Tick-borne encephalitis virus (TBEV) is a member of the Flavivirus genus, and belongs in the family Flaviviridae. The TBEV virion consists of three structural proteins, the envelope (E), membrane (M), and capsid (C) proteins, and a positive-sense single-stranded RNA genome. The NC is covered by the viral envelope that consists of host-derived lipids into which 180 copies of both M and E are embedded. The fundamental building block of the virion is a heterotetramer made up of two M–E dimers.

Here, we present the structure of a low-passage, European TBEV subtype (Kuutsalo-14) solved with cryo-EM and single-particle reconstruction to a resolution of 3.3 Å. The merged K3 datasets gave a final reconstruction with a resolution of 3.3 Å. The asymmetric unit contains three E–M heterodimers. Superimposition of the three E–M heterodimers within the asymmetric unit, based on the E protein ectodomains, indicated conformational differences between the M proteins located on the two-fold (chain D), three-fold (chain E), and five-fold (chain F) symmetry axes. The major conformational differences between the three M proteins arise due to the different locations of Asp23 and Ser24 that diverge by up to 2.8 Å at the Cα. Chains D and F twist towards each other and interact at the heterotetramer interfaces within the raft. One π-stacking interaction between Trp37 on each M protein, and two salt bridges between Lys40 and Glu33 stabilise the M protein interface. For each E–M dimer within the asymmetric unit, the reconstruction contained two densities not accounted for by the protein model. As phosphatidylcholine (PC) is the most common lipid species found in flavivirus virions, we built PC headgroups and the first four carbon atoms of each fatty acid tail. We built two N-acetylglucosamines (GlcNac) with core fucosylation (Fuc) at the first GlcNac into the density, which is consistent with the TBEV glycome and with previous flavivirus structures.

>SRCTHLENRDFVTGTQGTTRVTLVLELGGCVTITAEGKPSMDVWLDAIYQENPAKTREYCLHAKLSDTKVAARCPTMGPATLAEEHQGGTVCKRDQSDRGWGNHCGLFGKGSIVACVKAACEAKKKATGHVYDANKIVYTVKVEPHTGDYVAANETHSGRKTASFTVSSEKTILTMGEYGDVSLLCRVASGVDLAQTVILELDKTVEHLPTAWQVHRDWFNDLALPWKHEGAQNWNNAERLVEFGAPHAVKMDVYNLGDQTGVLLKALAGVPVAHIEGTKYHLKSGHVTCEVGLEKLKMKGLTYTMCDKTKFTWKRAPTDSGHDTVVMEVTFSGTKPCRIPVRAVAHGSPDVNVAMLITPNPTIENNGGGFIEMQLPPGDNIIYVGELSHQWFQKGSSIGRVFQKTKKGIERLTVIGEHAWDFGSAGGFLSSIGKAVHTVLGGAFNSIFGGVGFLPKLLLGVALAWLGLNMRNPTMSMSFLLAGGLVLAMTLGVGA[3x];>[3x]SVLIPSHAQGELTGRGHKWLEGDSLRTHLTRVEGWVWKNKLLALAMVTVVWLTLESVVTRVAVLVVLLCLAPVYA> DRVYIHPFHLLYYSKSTCAQLENPSVETLPEPTFEPVPIQAKTSPVDEKTLRDKLVLATEKLEAEDRQRAAQ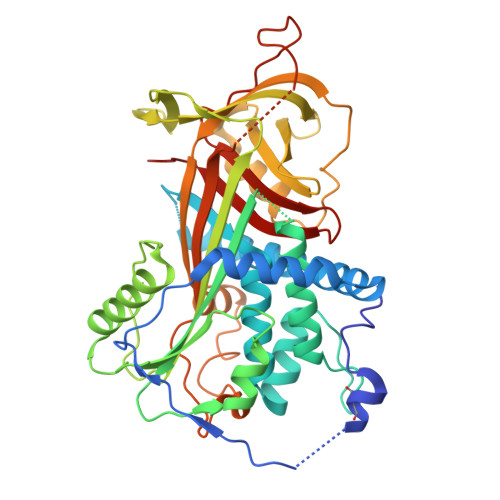VAMIANFVGFRMYKMLSEARGVASGAVLSPPALFGTLVSFYLGSLDPTASQLQVLLGVPVKEGDCTSRLDGHKVLTALQAVQGLLVTQGGSSSQTPLLQSTVVGLFTAPGLRLKQPFVESLGPFTPAIFPRSLDLSTDPVLAAQKINRFVQAVTGWKMNLPLEGVSTDSTLFFNTYVHFQGKMRGFSQLTGLHEFWVDNSTSVSVPMLSGTGNFQHWSDAQNNFSVTRVPLGESVTLLLIQPQCASDLDRVEVLVFQHDFLTWIKNPPPRAIRLTLPQLEIRGSYNLQDLLAQAKLSTLLGAEANLGKMGDTNPRVGEVLNSILLELQAGEEEQPTESAQQPGSPEVLDVTLSSPFLFAIYERDSGALHFLGRVDNPQNVV>[2x]MEPKLSKDTIIAAAFSLLEKSPTLEQLSMRKVAKQLGVQA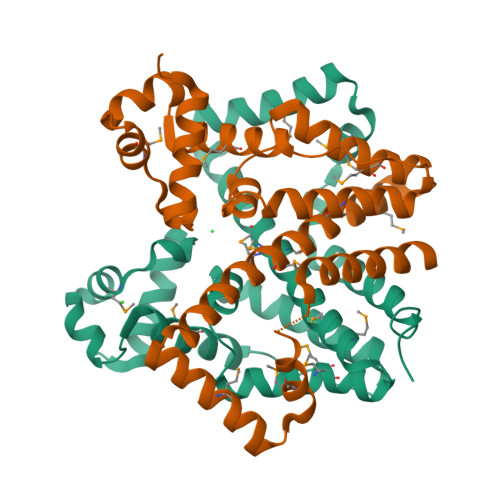PAIYWYFKNKQALLQSMAEAIEEHFQEPALCGEWYSDLLAFMENYYDLYQQFPCAVAIEIQTVPAYPQRLRHLNQMMGILREAGFSPEMTHLAVTSLQHLLFGMIMDATEEKQLVSQVLNGDDYLKEQVLHMKQYVSDNELTYMEESIQFRHSIHQKSAFIQAVKTYLDGLQADNTSSSK>MMKKADSVPTPAEAALAAQTALAADDSPMGDAARWAMGLLTSSGLPRPEDVAARFIPTFAAAGNFAETVREWRSKGPFTVRAYHPVAHKGWVVLSAPAGVRYILSLTLDSSGLIRILTLKPETVIPDMVTWNDVEETLHTPGVQHSVYAVRLTPDGHEVLHASAPERPMPTGSAYKLYLMRALVAEIEKGTVGWDEILTLTPELRSLPTGDMQDLPDGTRVTVRETAHKMIALSDNTGADLVADRLGREVVERSLAAAGHHDPSLMRPFLTSHEVFELGWGDPERRAEWVRQDEAGRRELLEKMAGVMTVRGSDLGATVHQLGIDWHMDAFDVVRVLEGLLQDSGRDTSGTVEEILTAYPGLLIDEERWRRVYFKAGSSPGVMMFCWLLQDH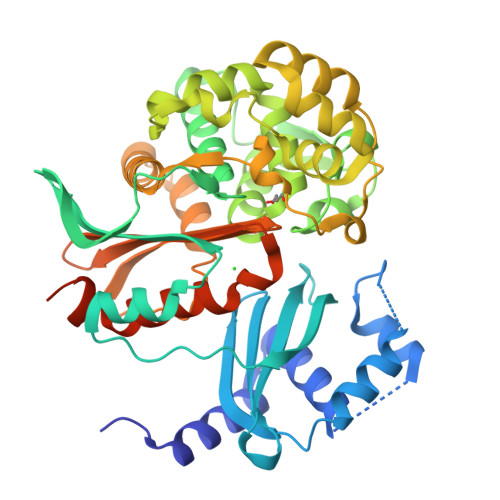AGISYVLVLRQSADEQRLIGDGLFLRGIGAKIIEAEAKLLSSGERRGAGTAAAGDDRASAGEAARR[2x]>MMRGSHHHHHTDPISYIIRKADSVNKALDSAVPLREPLKIHEAMRYSLLAGGKRVRPVLCIAACELVGGEESLAMPAACAVEMIHTMSLIHDDLPCMDNDDLRRGKPTNHKVYGEDVAVLAGDALLSFAFEHLASATSSEVSPARVVRAVGELAKAIGTEGLVAGQVVDISSEGLDLNNVGLEHLKFIHLHKTAALLEASAVLGGIIGGG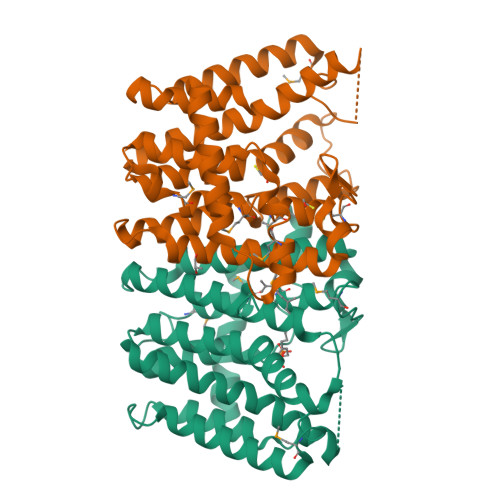SDEEIERLRKFARCIGLLFQVVDDILDVTKSSKLTYPKLMGLEKSREFAEKLNTEARDQLLGFDSDKVAPLLALANYIANRQN[2x]4-[ethoxy(oxidanyl)phosphoryl]-4-oxidanylidene-butanoic acid | C6 H11 O6 P 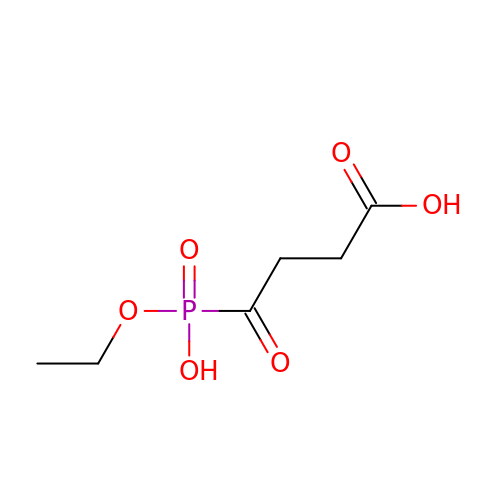| YEJCRQSMXRSGOQ-UHFFFAOYSA-N> GPRNLRVLLDTAIPPSFCDTVSSVLLDDFNMVSLIRTSPADSLATIKQDNAEIDIAITIDEELKISRFNQCVLGYTKAFVVAHPQHPLCNASLHSIASLANYRQISLGSRSGQHSNLLRPVSDKVLFVENFDDMLRLVEAGVGWGIAPHYFV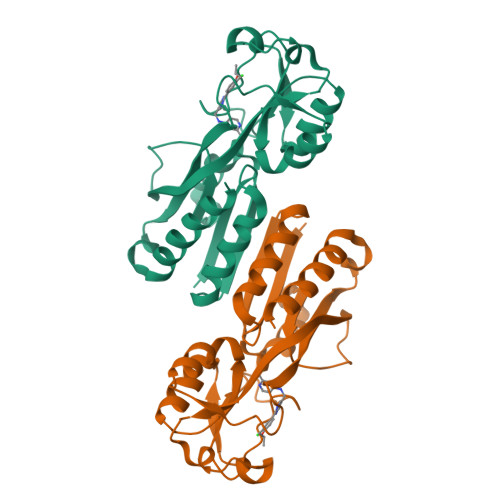EERLRNGTLAVLSELYEPGGIDTKVYCYYNTALESERSFLRFLESARQRLRELGRQRFDDAPAWQPSIVETAQRRSG1-(2-methylpropyl)imidazo[4,5-c]quinolin-4-amine | C14 H16 N4 | 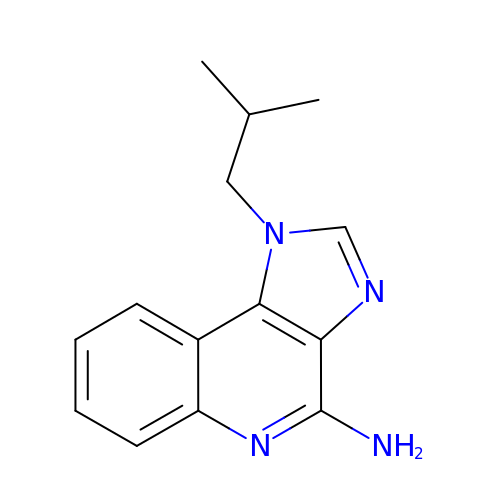DOUYETYNHWVLEO-UHFFFAOYSA-N> AALPDQSFLWNVFQRVDKDRSGVISDTELQQALSNGTWTPFNPVTVRSIISMFDRENKAGVNFSEFTGVWKYITDWQNVFRTYDRDNSGMIDKNELKQALSGAGYRLSDQFHDILIRKFDRQGRGQIAFDDFIQGCIVLQRLTDIFRRYDTDQDGWIQVSYEQYLSMVFSIV

ALG-2 (apoptosis-linked gene 2) is a 22-kDa protein of 191 amino acid residues containing five serially repetitive EF-hand-type helix-loop-helix Ca2+-binding motifs (EF1 to EF5) and it belongs to the penta-EF-hand (PEF) family, including the calpain small subunit, sorcin, grancalcin and peflin in mammals. ALG-2 (a gene product of PDCD6) belongs to the penta-EF-hand (PEF) protein family and Ca2+-dependently interacts with various intracellular proteins including mammalian Alix, an adaptor protein in the ESCRT system. X-ray crystal structures of various PEF proteins including ALG-2 have common features: the presence of eight α-helices and dimer formation via paired EF5s that are positioned in anti-parallel orientation. Binding of Ca2+ (or Zn2+) to EF3 enables the side chain of R125, present in the loop connecting EF3 and EF4, to move enough to make a primary hydrophobic pocket (Pocket 1) accessible to the critical PPYP motif found in Alix.

Surprisingly, however, the F122A mutant (ALG-2F122A, Phe substituted with Ala) exhibited an unexpected hyperactivity in Alix-binding. In the crystal structure of des3-20ALG-2F122A in the Zn2+-bound form, the axis of α5 inclined slightly outward from α4 and α7 (see Discussion section) (orange). On the other hand, NH2R125 in the structure of Zn2+-bound des3-20ALG-2F122A formed a hydrogen bond with OS120, and the side chain of R125 showed a configuration similar to that of wild-type ALG-2. In addition to two zinc ions found in EF1 and EF3 at the canonical coordination positions, one zinc ion that was coordinated at a non-canonical position was found in EF5 in the structure of Zn2+-bound des3-20ALG-2F122A. In this non-canonical EF-hand coordination, zinc ion was bonded to OD1D171 and OD2D173 in place of OD1D169 and OW175, respectively, at the x and -y positions. The bottom of Pocket 1 was supported by Y180 derived from a dimerizing counterpart molecule of ALG-2 (yellow). A wall formed by Gly121Phe122 in des3-20ALG-2/Ca2+-bound (green) disappeared in des3-23ALG-2ΔGF122/Ca2+-bound, and a surface structure represented by G123 was also changed (magenta) The continuous wall formed by 121-GFG-123 was maintained in Zn2+-bound des3-20ALG-2F122A (Figure 3D, orange: Gly121Ala122; magenta, G123). Comparison of the estimated angles formed by α4 (entering helix) and α5 (exiting helix) in EF3 between the structures of wild-type ALG-2 (θ = 54.5°) and des3-20ALG-2F122A (θ = 62.6°) in the Zn2+-bound forms indicates inclination of α5 by 8.1° away from α4, resulting in a shift in the position of the Cα atom of F122A for 2.0 Å. This more open conformation of the EF-hand motif in F122A mutant maintains distances or causes a small increase in distances between the Cα atoms of Y124 and T162 (facing Pocket 1) (WT, 9.9 Å; F122A, 10.1 Å) and between the Cα atoms of F122/A122 and Q159 (facing Pocket 2) (WT, 10.2 Å; F122A, 10.7 Å).>[2x]GPTLVPTKMQVTAPANISASAQTFEVACDYNGAIATLSDDGDMVGTAIVKDGKAIIKLNESIADETNLTLTVVGYNKVTVIKDVKVEGTS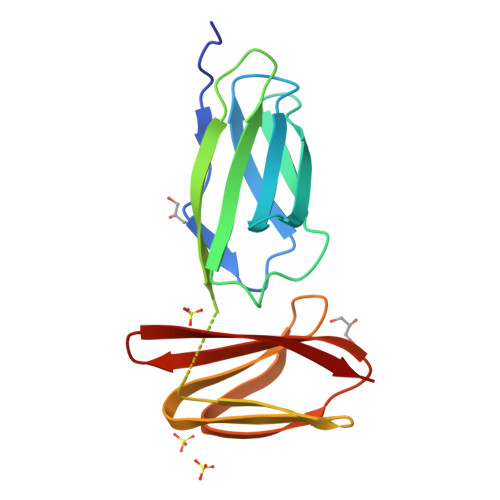HHHHHHIADVANDKPYTVAVSGKTITVESPAAGLTIFDMNGRRVATAKNRMVFEAQNGVYAVRIATEGKTYTEKVIVK1-(4-amino-1,2,5-oxadiazol-3-yl)-5-methyl-N-({3-[(5-methyl-4,5,6,7-tetrahydro[1,3]thiazolo[5,4-c]pyridin-2-yl)carbamoyl]phenyl}methyl)-1H-1,2,3-triazole-4-carboxamide | C21 H22 N10 O3 S | 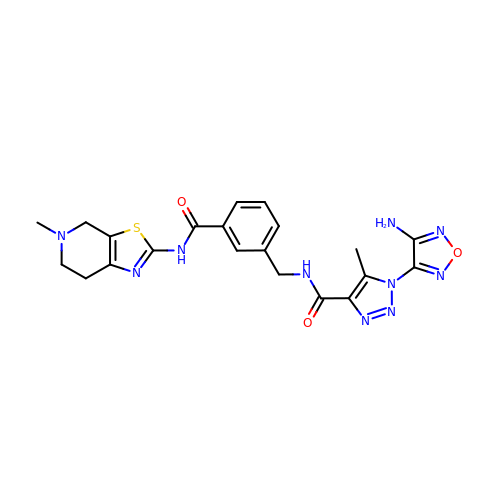UWMBHECVAPWYPU-UHFFFAOYSA-N> SLS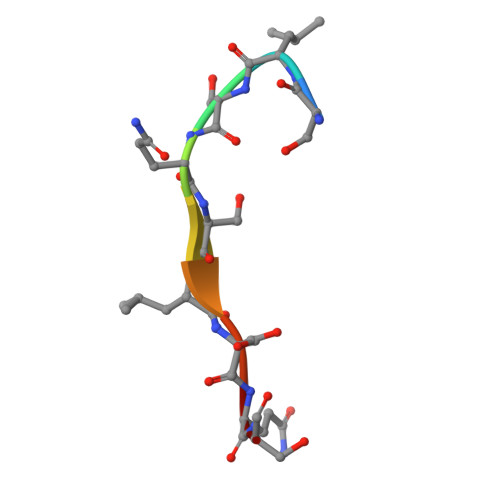QSLSQS> GAMGSEKSPSAQELKEQGNRLFVGRKYPEAAACYGRAITRNPLVAVYYTNRALCY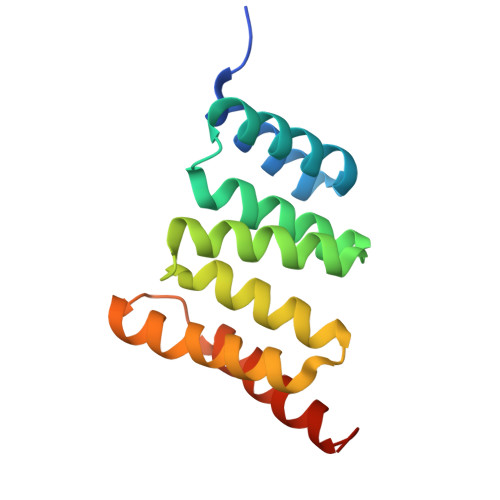LKMQQHEQALADCRRALELDGQSVKAHFFLGQCQLEMESYDEAIANLQRAYSLAKEQRLNFGDDIPSALRIAKKKRWNSIEERR> MTAIAPVITIDGPSGAGKGTLCKAMAEALQWHLLDSGAIYRVLALAALHHHVDVASEDALVPLASHLDVRFVSTNGNLEVILEGEDVSGEIRTQEVANAASQVAAFPRVREALLRRQRAFRELPGLIADGRDMGTVVFPDAPVKIFLDASSEER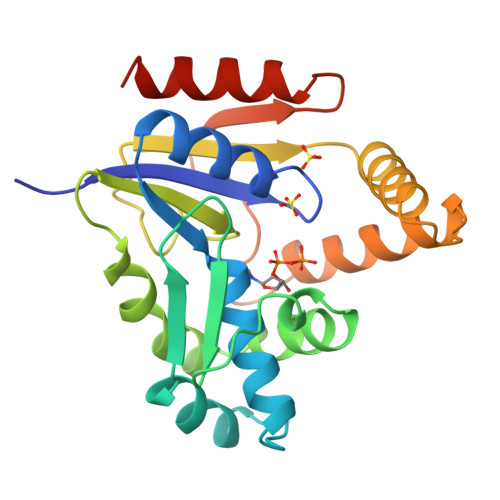AHRRMLQLQEKGFSVNFERLLAEIKERDDRDRNRAVAPLVPAADALVLDSTTLSIEQVIEKALQYARQKLALA>[2x]SVKFRDNFWGSKDAGMDALMSRTKSSLSVLESIDEFYAKRASIEREYASKLQELAASSADIPEVGSTLNNILSMRTETGSMAKAHEEVSQQINTELRNKIREYIDQTEQQKVVAANAIEELYQKKTALEIDLSKKKDAYEYSCNKLNSYMRQTKKMTGRELDKYNLKIRQAALAVKKMDAEYRETNELLLTVTREWIDRWTEVCDAFQHIEEYRLEFLKTNMWAYANIISTACVKDDESC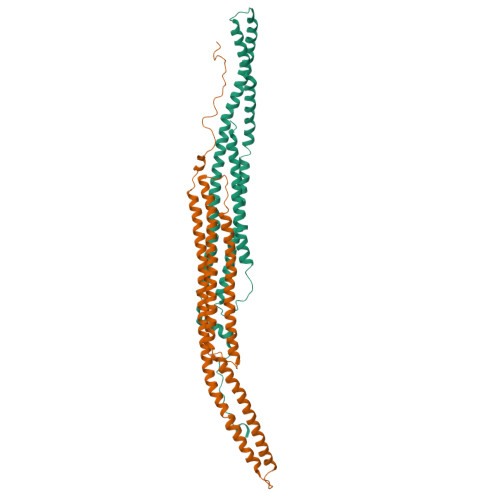EKIRLTLENTNIDEDITQMIQNEGTGTTIPPLPEFNDYFKENGLNYDIDQLISK4-[1-(5,8-difluoroquinolin-4-yl)-2-methyl-4-(4H-1,2,4-triazol-3-yl)-1H-benzimidazol-6-yl]-3-fluoropyridin-2-amine | C24 H15 F3 N8 | 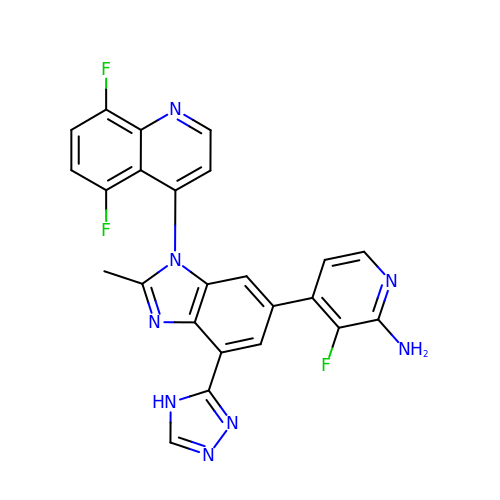SBVBUGSOYHJGGD-UHFFFAOYSA-N> PQIAAHVISEASSKTTSVLQWAEKGYYTMSNNLVTLENGKQLTVKR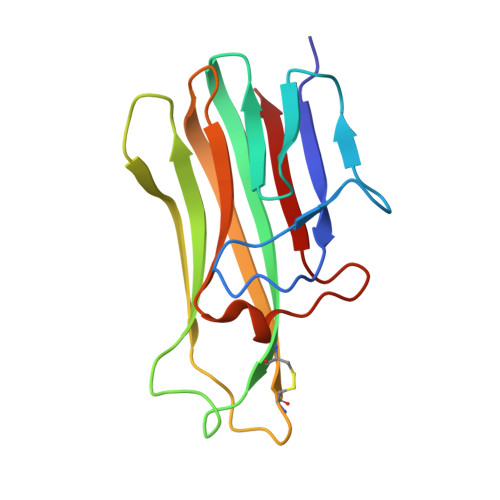QGLYYIYAQVTFCSNREASSQAPFIASLCLKSPGRFERILLRAANTHSSAKPCGQQSIHLGGVFELQPGASVFVNVTDPSQVSHGTGFTSFGLLKL>[2x]SNAMQKFIIHKGIACPLEYANIDTDQIIPKQFLLAVSKQGFGKHLFHDLRYLDDKESVLNMDFNLNKKEYQNSSILVSFENFGSGSSREHA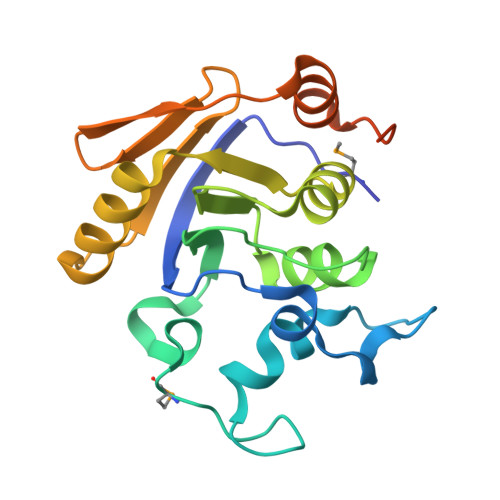PWALVDYGIRAIIAPSFADIFKNNALGNGLLTIELAKDEVLEIVDELKKSQDKNIEISLLEKRVFFKDKIFSFDLDDFHRICLLEGLDNIALTLKHEAQIKAYEKNSKSFLV2-(methylamino)-~{N}-[[3-[[2-(methylamino)ethanoylamino]methyl]phenyl]methyl]ethanamide 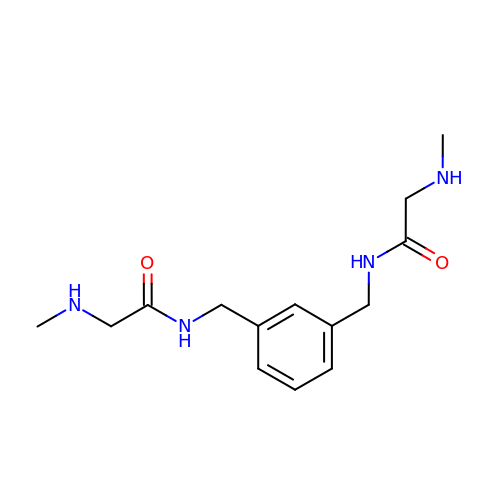| C14 H22 N4 O2 | CUFJKZFCOYUISD-UHFFFAOYSA-N>GPGYQDPNSAKLLQILNVRVVGSGERVVVLSHGFGTDQSAWSRVLPYLTRDHRVVLYDLVCAGSVNPDHFDFRRYDNLDAYVDDLLAILDALRIPRCAFVGHSVSAMIGILASIRRPDLFAKLVLIGASPRFLNDSDYHGGFELEEIQQVFDAMGANYSAWATGYAPLAVGADVPAAV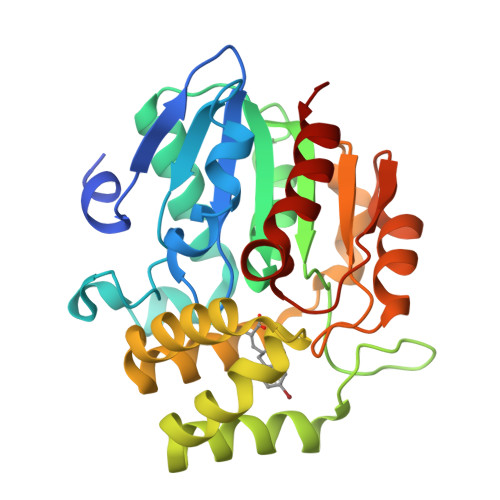QEFSRTLFNMRPDISLHVCQTVFKTDLRGVLGMVRAPCVVVQTTRDVSVPASVAAYLKAHLGGRTTVEFLQTEGHLPHLSAPSLLAQVLRRALARY[2x]>[9x]MAKTKGTASGRGGLGGQGAGGDVIEVGGAGQGGYGGLGSQGTSGRGGLGGQGAGGDVIEVGGAGQGGYGGLGSQGTSGRGGLGGQGAGGDVIEVGGAGQGGYGGLGSQGTSGRGGLGGQGAGGDVIEVGGAGQGGYGGLGSQGTSGRGGLGGQGAGGDVIEVGGAGQGGYGGLGSQGTSGRGGLGGQGAGGDVIEVGGAGQGGYGGLGSQGTSGRGGLGGQGAGGDVIEVGGAGQGGYGGLGSQGTSGRGGLGGQGAGGDVIEVGGAGQGGYGGLGSQGTSGRGGLGGQGAGGDVI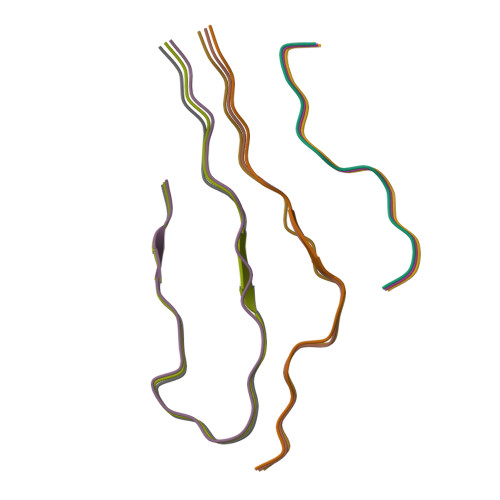EVGGAGQGGYGGLGSQGTSGRGGLGGQGAGGDVIEVGGAGQGGYGGLGSQGTSGRGGLGGQGAGGDVIEVGGAGQGGYGGLGSQGTSGRGGLGGQGAGGDVIEVGGAGQGGYGGLGSQGTSGRGGLGGQGAGGDVIEVGGAGQGGYGGLGSQGTSGRGGLGGQGAGGDVIEVGGAGQGGYGGLGSQGTSGRGGLGGQGAGGDVIEVGGAGQGGYGGLGSQGTSGRGGLGGQGAGGDVIEVGGAGQGGYGGLGSQGTSSGHHHHHHHHHH>[8x]IIDGAPCARGSHPWQVALLSGNQLHCGGVLVNERWVLTAAHCKMNEYTVHLGSDTLGDRRAQRIKASKSFRHPGYSTQTHVNDLMLVKLNSQARLSSMVK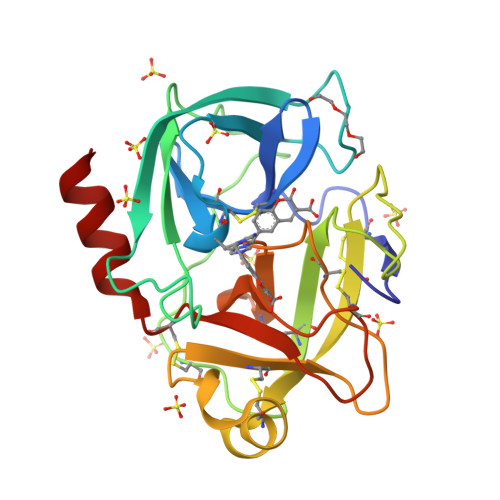KVRLPSRCEPPGTTCTVSGWGTTTSPDVTFPSDLMCVDVKLISPQDCTKVYKDLLENSMLCAGIPDSKKNACNGDSGGPLVCRGTLQGLVSWGTFPCGQPNDPGVYTQVCKFTKWINDTMKKHR>GAMETITVPTPIKQIFSDDAFAETIKDNLKKKSVTDAVTQNELNSIDQIIANNSDIKSVQGIQYLPNLTSLNLSNNQITDISPIQYLPNVTKLFLNGNKLTDIKPLANLKNLGWLFLDENKVKDLSSLKDLKKLKSLSLEHNGISDINGLVHLPQLESLYLGNNKITDITVLSRLTKLDTLSLEDNQISDIVPLAGLTKLQNLYLSKNHISDLRALAGLKNLDVLELFSQECLNKPINHQSNLVVPNTVKNTDGSLVTPEIISD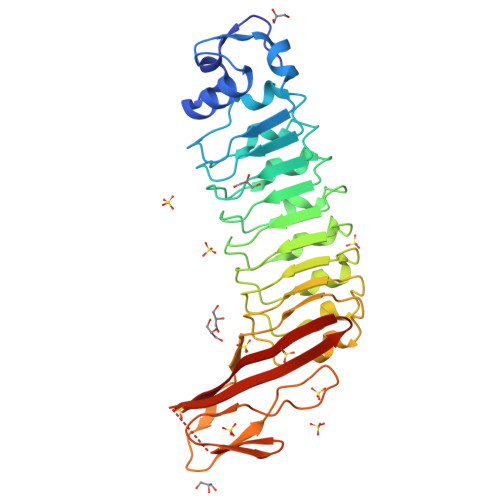DGDYEKPNVKWHLPEFTNEVSFIFYQPVTIGKAKARFHGRVTQPLKE[3x]>[6x]MGSDKIHHHHHHMAFFDLPLEELKKYRPERYEEKDFDEFWEETLAESEKFPLDPVFERMESHLKTVEAYDVTFSGYRGQRIKGWLLVPKLEEEKLPCVVQYIGYNGGRGFPHDWLFWPSMGYICFVMDTRGQGSGWLKGDTPDYPEGPVDPQYPGFMTRGILDPRTYYYRR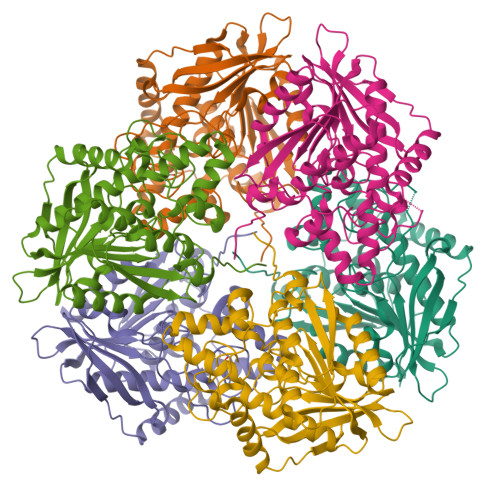VFTDAVRAVEAAASFPQVDQERIVIAGGSQGGGIALAVSALSKKAKALLCDVPFLCHFRRAVQLVDTHAYAEITNFLKTHRDKEEIVFRTLSYFDGVNFAARAKIPALFSVGLMDNICPPSTVFAAYNYYAGPKEIRIYPYNNHEGGGSFQAVEQVKFLKKLFEKG>[2x]MHHHHHHENLYFQGRFDNKVVVITGAGNGMGEAAARRFSAEGAIVVLADWAKEAVDKVAASLPKGRAMAVHIDVSDHVAVEKMMNEVAEKLGRIDVLLNNAGVHVAGSVLETSIDDWRRIAGVDIDGVVFCSKFALPHLLKTKGCIVNTASVSGLGGDWGAAYYCAAKGAVVNLTRAMALDHGGDGVRINSVCPSLVKTNMTNGWPQEIRDKFNERIALGRA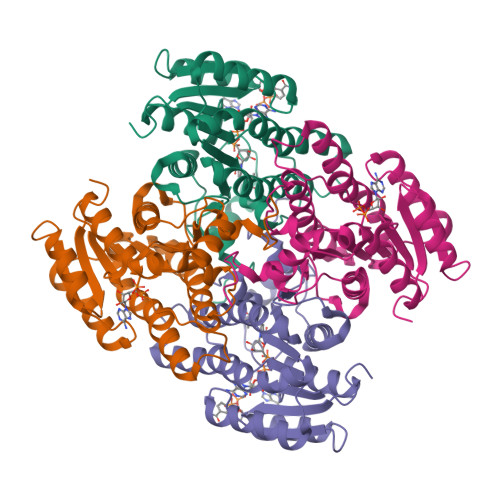AEPEEVAAVMAFLASDDASFINGANIPVDGGATASDGQPKIV> MKHMPRKMYSCAFETTTKVEDCRVWAYGYMNIEDHSEYKIGNSLDEFMAWV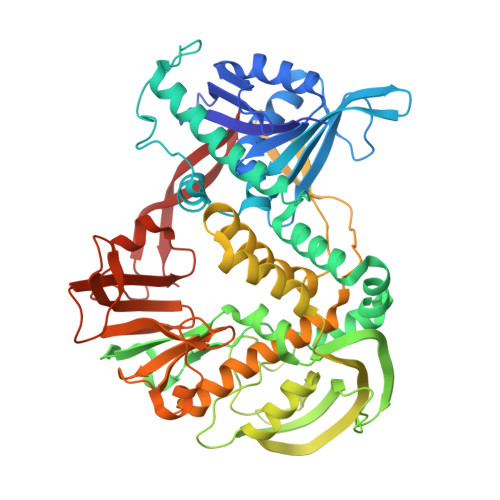LKVQADLYFHNLKFAGAFIINWLERNGFKWSADGLPNTYNTIISRMGQWYMIDICLGYKGKRKIHTVIYDSLKKLPFPVKKIAKDFKLTVLKGDIDYHKERPVGYKITPEEYAYIKNDIQIIAEALLIQFKQGLDRMTAGSDSLKGFKDIITTKKFKKVFPTLSLGLDKEVRYAYRGGFTWLNDRFKEKEIGEGMVFDVNSLYPAQMYSRLLPYGEPIVFEGKYVWDEDYPLHIQHIRCEFELKEGYIPTIQIKRSRFYKGNEYLKSSGGEIADLWLSNVDLELMKEHYDLYNVEYISGLKFKATTGLFKDFIDKWTYIKTTSEGAIKQLAKLMLNSLYGKFASNPDVTGKVPYLKENGALGFRLGEEETKDPVYTPMGVFITAWARYTTITAAQACYDRIIYCDTDSIHLTGTEIPDVIKDIVDPKKLGYWAHESTFKRAKYLRQKTYIQDIYMKEVDGKLVEGSPDDYTDIKFSVKCAGMTDKIKKEVTFENFKVGFSRKMKPKPVQVPGGVVLVDDTFTIK>[2x]C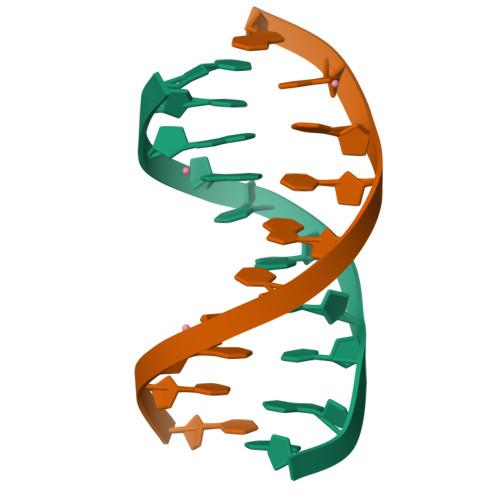CGGTACCGG>[4x]MERPQPDSMPQDLSEALKEATKEVHTQAENAEFMRNFQKGQVTRDGFKLVMASLYHIYVA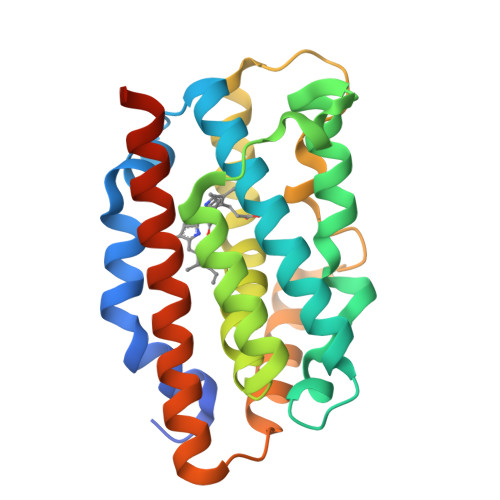LEEEIERNKESPVFAPVYFPEELHRKAALEQDLAFWYGPRWQEVIPYTPAMQRYVKRLHEVGRTEPELLVAHAYTRYLGDLSGGQVLKKIAQKALDLPSSGEGLAFFTFPNIASATKFKQLYRSRMNSLEMTPAVRQRVIEEAKTAFLLNIQLFEELQELLTHDTKDQSPSRA>MEPAMEPETLEARINRATNPLNKELDWASINGFCEQLNEDFEGPPLATRLLAHKIQSPQEWEAIQALTVLETCMKSCGKRFHDEVGKFRFLNELIKVVSPKYLGSRTSEKVKNKILELLYSWTVGLPEEVKIAEAYQMLKKQGIVKS[2x]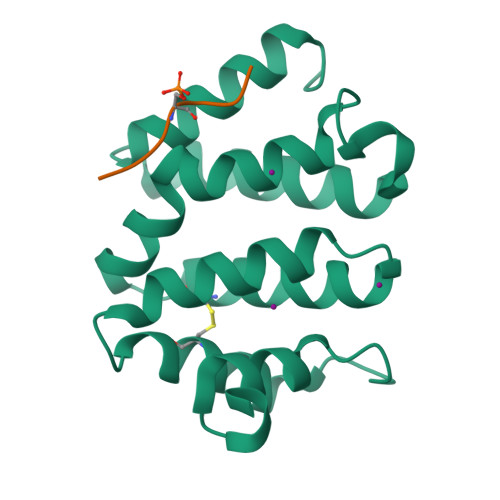;>[2x]HDDFADDISLLK> MSASFVPNGASLEDCHCNLFCLADLTGIKWKKYVWQGPTSAPILFPVTEEDPILSSFSRCLKADVLGVWRRDQRPGRRELWIFWWGEDPSFADLIHHDLSEEEDGVWENGLSYECRTLLFKAVHNLLERCLMNRNFVRIGKWFVKPYEKDEKPINKSEHLSCSFTFFLHGDSNVCTSVEINQHQPVYLLSEEHITLAQQSNSPFQVILCPFGLNGTLTGQAFKMSDSATKKLIGEWKQFYPISCCLKEMSEEKQEDMDWEDDSLAAVEVLVAGVRMIYPACFVLVPQSDIPTPSPVGSTHCSSSCLGVHQVPASTRDPAMSSVTLTPPTSPEEVQTVDPQSVQKWVKFSSVSDGFNSDSTSHHGGKIPRKLANHVVDRVWQECNMNRAQNKRKYSASSGGLCEEATAAKVASWDFVEATQRTNCSCLRHKNLKSRNAGQQGQAPSLGQQQQILPKHKTNEKQEKSEKPQKRPLTPFHHRVSVSDDVGMDADSASQRLVISAPDSQVRFSNIRTNDVAKTPQMHGTEMANSPQPPPLSPHPCDVVDEGVTKTPSTPQSQHFYQMPTPDPLVPSKPMEDRIDSLSQSFPPQYQEAVEPTVYVGTAVNLEEDEANIAWKYYKFPKKKDVEFLPPQLPSDKFKDDPVGPFGQESVTSVTELMVQCKKPLKVSDELVQQYQIKNQCLSAIASDAEQEPKIDPYAFVEGDEEFLFPDKKDRQNSEREAGKKHKVEDGTSSVTVLSHEEDAMSLFSPSIKQDAPRPTSHARPPSTSLIYDSDLAVSYTDLDNLFNSDEDELTPGSKKSANGSDDKASCKESKTGNLDPLSCISTADLHKMYPTPPSLEQHIMGFSPMNMNNKEYGSMDTTPGGTVLEGNSSSIGAQFKIEVDEGFCSPKPSEIKDFSYVYKPENCQILVGCSMFAPLKTLPSQYLPPIKLPEECIYRQSWTVGKLELLSSGPSMPFIKEGDGSNMDQEYGTAYTPQTHTSFGMPPSSAPPSNSGAGILPSPSTPRFPTPRTPRTPRTPRGAGGPASAQGSVKYENSDLYSPASTPSTCRPLNSVEPATVPSIPEAHSLYVNLILSESVMNLFKDCNFDSCCICVCNMNIKGADVGVYIPDPTQEAQYRCTCGFSAVMNRKFGNNSGLFLEDELDIIGRNTDCGKEAEKRFEALRATSAEHVNGGLKESEKLSDDLILLLQDQCTNLFSPFGAADQDPFPKSGVISNWVRVEERDCCNDCYLALEHGRQFMDNMSGGKVDEALVKSSCLHPWSKRNDVSMQCSQDILRMLLSLQPVLQDAIQKKRTVRPWGVQGPLTWQQFHKMAGRGSYGTDESPEPLPIPTFLLGYDYDYLVLSPFALPYWERLMLEPYGSQRDIAYVVLCPENEALLNGAKSFFRDLTAIYESCRLGQHRPVSRLLTDGIMRVGSTASKKLSEKLVAEWFSQAADGNNEAFSKLKLYAQVCRYDLGPYLASLPLDSSLLSQPNLVAPTSQSLITPPQMTNTGNANTPSATLASAASSTMTVTSGVAISTSVATANSTLTTASTSSSSSSNLNSGVSSNKLPSFPPFGSMNSNAAGSMSTQANTVQSGQLGGQQTSALQTAGISGESSSLPTQPHPDVSESTMDRDKVGIPTDGDSHAVTYPPAIVVYIIDPFTYENTDESTNSSSVWTLGLLRCFLEMVQTLPPHIKSTVSVQIIPCQYLLQPVKHEDREIYPQHLKSLAFSAFTQCRRPLPTSTNVKTLTGFGPGLAMETALRSPDRPECIRLYAPPFILAPVKDKQTELGETFGEAGQKYNVLFVGYCLSHDQRWILASCTDLYGELLETCIINIDVPNRARRKKSSARKFGLQKLWEWCLGLVQMSSLPWRVVIGRLGRIGHGELKDWSCLLSRRNLQSLSKRLKDMCRMCGISAADSPSILSACLVAMEPQGSFVIMPDSVSTGSVFGRSTTLNMQTSQLNTPQDTSCTHILVFPTSASVQVASATYTTENLDLAFNPNNDGADGMGIFDLLDTGDDLDPDIINILPASPTGSPVHSPGSHYPHGGDAGKGQSTDRLLSTEPHEEVPNILQQPLALGYFVSTAKAGPLPDWFWSACPQAQYQCPLFLKASLHLHVPSVQSDELLHSKHSHPLDSNQTSDVLRFVLEQYNALSWLTCDPATQDRRSCLPIHFVVLNQLYNFIMNML;> MKAQGETEESEKLSKMSSLLERLHAKFNQNRPWSETIKLVRQVMEKRVVMSSGGHQHLVSCLETLQKALKVTSLPAMTDRLESIARQNGLGSHLSASGTECYITSDMFYVEVQLDPAGQLCDVKVAHHGENPVSCPELVQQLREKNFDEFSKHLKGLVNLYNLPGDNKLKTKMYLALQSLEQDLSKMAIMYWKATNAGPLDKILHGSVGYLTPRSGGHLMNLKYYVSPSDLLDDKTASPIILHENNVSRSLGMNASVTIEGTSAVYKLPIAPLIMGSHPVDNKWTPSFSSITSANSVDLPACFFLKFPQPIPVSRAFVQKLQNCTGIPLFETQPTYAPLYELITQFELSKDPDPIPLNHNMRFYAALPGQQHCYFLNKDAPLPDGRSLQGTLVSKITFQHPGRVPLILNLIRHQVAYNTLIGSCVKRTILKEDSPGLLQFEVCPLSESRFSVSFQHPVNDSLVCVVMDVQDSTHVSCKLYKGLSDALICTDDFIAKVVQRCMSIPVTMRAIRRKAETIQADTPALSLIAETVEDMVKKNLPPASSPGYGMTTGNNPMSGTTTPTNTFPGGPITTLFNMSMSIKDRHESVGHGEDFSKVSQNPILTSLLQITGNGGSTIGSSPTPPHHTPPPVSSMAGNTKNHPMLMNLLKDNPAQDFSTLYGSSPLERQNSSSGSPRMEICSGSNKTKKKKSSRLPPEKPKHQTEDDFQRELFSMDVDSQNPIFDVNMTADTLDTPHITPAPSQCSTPPTTYPQPVPHPQPSIQRMVRLSSSDSIGPDVTDILSDIAEEASKLPSTSDDCPAIGTPLRDSSSSGHSQSTLFDSDVFQTNNNENPYTDPADLIADAAGSPSSDSPTNHFFHDGVDFNPDLLNSQSQSGFGEEYFDESSQSGDNDDFKGFASQALNTLGVPMLGGDNGETKFKGNNQADTVDFSIISVAGKALAPADLMEHHSGSQGPLLTTGDLGKEKTQKRVKEGNGTSNSTLSGPGLDSKPGKRSRTPSNDGKSKDKPPKRKKADTEGKSPSHSSSNRPFTPPTSTGGSKSPGSAGRSQTPPGVATPPIPKITIQIPKGTVMVGKPSSHSQYTSSGSVSSSGSKSHHSHSSSSSSSASTSGKMKSSKSEGSSSSKLSSSMYSSQGSSGSSQSKNSSQSGGKPGSSPITKHGLSSGSSSTKMKPQGKPSSLMNPSLSKPNISPSHSRPPGGSDKLASPMKPVPGTPPSSKAKSPISSGSGGSHMSGTSSSSGMKSSSGLGSSGSLSQKTPPSSNSCTASSSSFSSSGSSMSSSQNQHGSSKGKSPSRNKKPSLTAVIDKLKHGVVTSGPGGEDPLDGQMGVSTNSSSHPMSSKHNMSGGEFQGKREKSDKDKSKVSTSGSSVDSSKKTSESKNVGSTGVAKIIISKHDGGSPSIKAKVTLQKPGESSGEGLRPQMASSKNYGSPLISGSTPKHERGSPSHSKSPAYTPQNLDSESESGSSIAEKSYQNSPSSDDGIRPLPEYSTEKHKKHKKEKKKVKDKDRDRDRDKDRDKKKSHSIKPESWSKSPISSDQSLSMTSNTILSADRPSRLSPDFMIGEEDDDLMDVALIGN;> MAASSSGEKEKERLGGGLGVAGGNSTRERLLSALEDLEVLSRELIEMLAISRNQKLLQAGEENQVLELLIHRDGEFQELMKLALNQGKIHHEMQVLEKEVEKRDSDIQQLQKQLKEAEQILATAVYQAKEKLKSIEKARKGAISSEEIIKYAHRISASNAVCAPLTWVPGDPRRPYPTDLEMRSGLLGQMNNPSTNGVNGHLPGDALAAGRLPDVLAPQYPWQSNDMSMNMLPPNHSSDFLLEPPGHNKENEDDVEIMSTDSSSSSSESD;> MAAVDIRDNLLGISWVDSSWIPILNSGSVLDYFSERSNPFYDRTCNNEVVKMQRLTLEHLNQMVGIEYILLHAQEPILFIIRKQQRQSPAQVIPLADYYIIAGVIYQAPDLGSVINSRVLTAVHGIQSAFDEAMSYCRYHPSKGYWWHFKDHEEQDKVRPKAKRKEEPSSIFQRQRVDALLLDLRQKFPPKFVQLKPGEKPVPVDQTKKEAEPIPETVKPEEKETTKNVQQTVSAKGPPEKRMRLQ;> MGEPQQVSALPPPPMQYIKEYTDENIQEGLAPKPPPPIKDSYMMFGNQFQCDDLIIRPLESQGIERLHPMQFDHKKELRKLNMSILINFLDLLDILIRSPGSIKREEKLEDLKLLFVHVHHLINEYRPHQARETLRVMMEVQKRQRLETAERFQKHLERVIEMIQNCLASLPDDLPHSEAGMRVKTEPMDADDSNNCTGQNEHQRENSGHRRDQIIEKDAALCVLIDEMNERP;> MQREEKQLEASLDALLSQVADLKNSLGSFICKLENEYGRLTWPSVLDSFALLSGQLNTLNKVLKHEKTPLFRNQVIIPLVLSPDRDEDLMRQTEGRVPVFSHEVVPDHLRTKPDPEVEEQEKQLTTDAARIGADAAQKQIQSLNKMCSNLLEKISKEERESESGGLRPNKQTFNPTDTNALVAAVAFGKGLSNWRPSGSSGPGQAGQPGAGTILAGTSGLQQVQMAGAPSQQQPMLSGVQMAQAGQPGKMPSGIKTNIKSASMHPYQR;> MASAGVAAGRQAEDVLPPTSDQPLPDTKPLPPPQPPPVPAPQPQQSPAPRPQSPARAREEENYSFLPLVHNIIKCMDKDSPEVHQDLNALKSKFQEMRKLISTMPGIHLSPEQQQQQLQSLREQVRTKNELLQKYKSLCMFEIPKE;> MAEKFDHLEEHLEKFVENIRQLGIIVSDFQPSSQAGLNQKLNFIVTGLQDIDKCRQQLHDITVPLEVFEYIDQGRNPQLYTKECLERALAKNEQVKGKIDTMKKFKSLLIQELSKVFPEDMAKYRSIRGEDHPPS;> MATYSLANERLRALEDIEREIGAILQNAGTVILELSKEKTNERLLDRQAAAFTASVQHVEAELSAQIRYLTQVATGQPHEGSSYSSRKDCQMALKRVDYARLKLSDVARTCEQMLEN;> MAPVQLENHQLVPPGGGGGGSGGPPSAPAPPPPGAAVAAAAAAAASPGYRLSTLIEFLLHRAYSELMVLTDLLPRKSDVERKIEIVQFASRTRQLFVRLLALVKWANNAGKVEKCAMISSFLDQQAILFVDTADRLASLARDALVHARLPSFAIPYAIDVLTTGSYPRLPTCIRDKIIPPDPITKIEKQATLHQLNQILRHRLVTTDLPPQLANLTVANGRVKFRVEGEFEATLTVMGDDPDVPWRLLKLEILVEDKETGDGRALVHSMQISFIHQLVQSRLFADEKPLQDMYNCLHSFCLSLQLEVLHSQTLMLIRERWGDLVQVERYHAGKCLSLSVWNQQVLGRKTGTASVHKVTIKIDENDVSKPLQIFHDPPLPASDSKLVERAMKIDHLSIEKLLIDSVHARAHQKLQELKAILRGFNANENSSIETALPALVVPILEPCGNSECLHIFVDLHSGMFQLMLYGLDQATLDDMEKSVNDDMKRIIPWIQQLKFWLGQQRCKQSIKHLPTISSETLQLSNYSTHPIGNLSKNKLFIKLTRLPQYYIVVEMLEVPNKPTQLSYKYYFMSVNAADREDSPAMALLLQQFKENIQDLVFRTKTGKQTRTNAKRKLSDDPCPVESKKTKRAGEMCAFNKVLAHFVAMCDTNMPFVGLRLELSNLEIPHQGVQVEGDGFSHAIRLLKIPPCKGITEETQKALDRSLLDCTFRLQGRNNRTWVAELVFANCPLNGTSTREQGPSRHVYLTYENLLSEPVGGRKVVEMFLNDWNSIARLYECVLEFARSLPDIPAHLNIFSEVRVYNYRKLILCYGTTKGSSISIQWNSIHQKFHISLGTVGPNSGCSNCHNTILHQLQEMFNKTPNVVQLLQVLFDTQAPLNAINKLPTVPMLGLTQRTNTAYQCFSILPQSSTHIRLAFRNMYCIDIYCRSRGVVAIRDGAYSLFDNSKLVEGFYPAPGLKTFLNMFVDSNQDARRRSVNEDDNPPSPIGGDMMDSLISQLQPPPQQQPFPKQPGTSGAYPLTSPPTSYHSTVNQSPSMMHTQSPGNLHAASSPSGALRAPSPASFVPTPPPSSHGISIGPGASFASPHGTLDPSSPYTMVSPSGRAGNWPGSPQVSGPSPAARMPGMSPANPSLHSPVPDASHSPRAGTSSQTMPTNMPPPRKLPQRSWAASIPTILTHSALNILLLPSPTPGLVPGLAGSYLCSPLERFLGSVIMRRHLQRIIQQETLQLINSNEPGVIMFKTDALKCRVALSPKTNQTLQLKVTPENAGQWKPDELQVLEKFFETRVAGPPFKANTLIAFTKLLGAPTHILRDCVHIMKLELFPDQATQLKWNVQFCLTIPPSAPPIAPPGTPAVVLKSKMLFFLQLTQKTSVPPQEPVSIIVPIIYDMASGTTQQADIPRQQNSSVAAPMMVSNILKRFAEMNPPRQGECTIFAAVRDLMANLTLPPGGRP;> MDVSGQETDWRSTAFRQKLVSQIEDAMRKAGVAHSKSSKDMESHVFLKAKTRDEYLSLVARLIIHFRDIHNKKSQASVSDPMNALQSLTGGPAAGAAGIGMPPRGPGQSLGGMGSLGAMGQPMSLSGQPPPGTSGMAPHSMAVVSTATPQTQLQLQQVALQQQQQQQQFQQQQQAALQQQQQQQQQQQFQAQQSAMQQQFQAVVQQQQQLQQQQQQQQHLIKLHHQNQQQIQQQQQQLQRIAQLQLQQQQQQQQQQQQQQQQALQAQPPIQQPPMQQPQPPPSQALPQQLQQMHHTQHHQPPPQPQQPPVAQNQPSQLPPQSQTQPLVSQAQALPGQMLYTQPPLKFVRAPMVVQQPPVQPQVQQQQTAVQTAQAAQMVAPGVQMITEALAQGGMHIRARFPPTTAVSAIPSSSIPLGRQPMAQVSQSSLPMLSSPSPGQQVQTPQSMPPPPQPSPQPGQPSSQPNSNVSSGPAPSPSSFLPSPSPQPSQSPVTARTPQNFSVPSPGPLNTPVNPSSVMSPAGSSQAEEQQYLDKLKQLSKYIEPLRRMINKIDKNEDRKKDLSKMKSLLDILTDPSKRCPLKTLQKCEIALEKLKNDMAVPTPPPPPVPPTKQQYLCQPLLDAVLANIRSPVFNHSLYRTFVPAMTAIHGPPITAPVVCTRKRRLEDDERQSIPSVLQGEVARLDPKFLVNLDPSHCSNNGTVHLICKLDDKDLPSVPPLELSVPADYPAQSPLWIDRQWQYDANPFLQSVHRCMTSRLLQLPDKHSVTALLNTWAQSVHQACLSAA;> MCDLRRPAAGGMMDLAYVCEWEKWSKSTHCPSVPLACAWSCRNLIAFTMDLRSDDQDLTRMIHILDTEHPWDLHSIPSEHHEAITCLEWDQSGSRLLSADADGQIKCWSMADHLANSWESSVGSLVEGDPIVALSWLHNGVKLALHVEKSGASSFGEKFSRVKFSPSLTLFGGKPMEGWIAVTVSGLVTVSLLKPSGQVLTSTESLCRLRGRVALADIAFTGGGNIVVATADGSSASPVQFYKVCVSVVSEKCRIDTEILPSLFMRCTTDLNRKDKFPAITHLKFLARDMSEQVLLCASSQTSSIVECWSLRKEGLPVNNIFQQISPVVGDKQPTILKWRILSATNDLDRVSAVALPKLPISLTNTDLKVASDTQFYPGLGLALAFHDGSVHIVHRLSLQTMAVFYSSAAPRPVDEPAMKRPRTAGPAVHLKAMQLSWTSLALVGIDSHGKLSVLRLSPSMGHPLEVGLALRHLLFLLEYCMVTGYDWWDILLHVQPSMVQSLVEKLHEEYTRQTAALQQVLSTRILAMKASLCKLSPCTVTRVCDYHTKLFLIAISSTLKSLLRPHFLNTPDKSPGDRLTEICTKITDVDIDKVMINLKTEEFVLDMNTLQALQQLLQWVGDFVLYLLASLPNQGSLLRPGHSFLRDGTSLGMLRELMVVIRIWGLLKPSCLPVYTATSDTQDSMSLLFRLLTKLWICCRDEGPASEPDEALVDECCLLPSQLLIPSLDWLPASDGLVSRLQPKQPLRLQFGRAPTLPGSAATLQLDGLARAPGQPKIDHLRRLHLGACPTEECKACTRCGCVT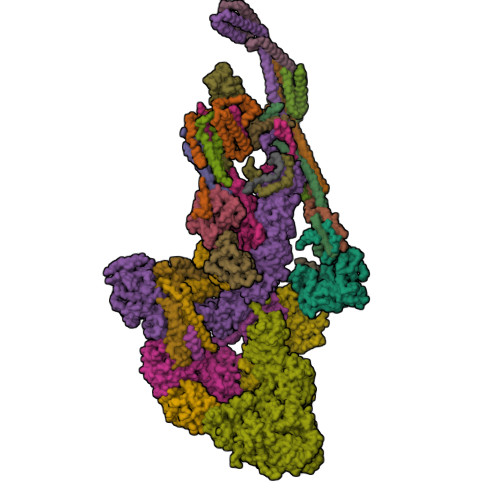MLKSPNRTTAVKQWEQRWIKNCLAVEGRGPDACVTSRASEEAPAFVQLGPQSTHHSPRTPRSLDHLHPEDRP;> MSGVRAVRISIESACEKQVHEVGLDGTETYLPPLSMSQNLARLAQRIDFSQGSGSEEEEAAGTEGDAQEWPGAGSSADQDDEEGVVKFQPSLWPWDSVRNNLRSALTEMCVLYDVLSIVRDKKFMTLDPVSQDALPPKQNPQTLQLISKKKSLAGAAQILLKGAERLTKSVTENQENKLQRDFNSELLRLRQHWKLRKVGDKILGDLSYRSAGSLFPHHGTFEVIKNTDLDLDKKIPEDYCPLDVQIPSDLEGSAYIKVSIQKQAPDIGDLGTVNLFKRPLPKSKPGSPHWQTKLEAAQNVLLCKEIFAQLSREAVQIKSQVPHIVVKNQIISQPFPSLQLSISLCHSSNDKKSQKFATEKQCPEDHLYVLEHNLHLLIREFHKQTLSSIMMPHPASAPFGHKRMRLSGPQAFDKNEINSLQSSEGLLEKIIKQAKHIFLRSRAAATIDSLASRIEDPQIQAHWSNINDVYESSVKVLITSQGYEQICKSIQLQLNIGVEQIRVVHRDGRVITLSYQEQELQDFLLSQMSQHQVHAVQQLAKVMGWQVLSFSNHVGLGPIESIGNASAITVASPSGDYAISVRNGPESGSKIMVQFPRNQCKDLPKSDVLQDNKWSHLRGPFKEVQWNKMEGRNFVYKMELLMSALSPCLL;> MEAPPVTMMPVTGGTINMMEYLLQGSVLDHSLESLIHRLRGLCDNMEPETFLDHEMVFLLKGQQASPFVLRARRSMDRAGAPWHLRYLGQPEMGDKNRHALVRNCVDIATSENLTDFLMEMGFRMDHEFVAKGHLFRKGIMKIMVYKIFRILVPGNTDSTEALSLSYLVELSVVAPAGQDMVSDDMKNFAEQLKPLVHLEKIDPKRLM;> MGVTCVSQMPVAEGKSVQQTVELLTRKLEMLGAEKQGTFCVDCETYHTAASTLGSQGQTGKLMYVMHNSEYPLSCFALFENGPCLIADTNFDVLMVKLKGFFQSAKASKIETRGTRYQYCDFLVKVGTVTMGPSARGISVEVEYGPCVVASDCWSLLLEFLQSFLGSHTPGAPAVFGNRHDAVYGPADTMVQYMELFNKIRKQQQVPVAGIR;> MADRLTQLQDAVNSLADQFCNAIGVLQQCGPPASFNNIQTAINKDQPANPTEEYAQLFAALIARTAKDIDVLIDSLPSEESTAALQAASLYKLEEENHEAATCLEDVVYRGDMLLEKIQSALADIAQSQLKTRSGTHSQSLPDS;> MAQQRALPQSKETLLQSYNKRLKDDIKSIMDNFTEIIKTAKIEDETQVSRATQGEQDNYEMHVRAANIVRAGESLMKLVSDLKQFLILNDFPSVNEAIDQRNQQLRTLQEECDRKLITLRDEISIDLYELEEEYYSSSSSLCEANDLPLCEAYGRLDLDTDSADGLSAPLLASPEPSAGPLQVAAPAHSHAGGPGPTEHA;> METQLQSIFEEVVKTEVIEEAFPGMFMDTPEDEKTKLISCLGAFRQFWGGLSQESHEQCIQWIVKFIHGQHSPKRISFLYDCLAMAVETGLLPPRLVCESLINSDTLEWERTQLWALTFKLVRKIIGGVDYKGVRDLLKVILEKILTIPNTVSSAVVQQLLAAREVIAYILERNACLLPAYFAVTEIRKLYPEGKLPHWLLGNLVSDFVDTFRPTARINSICGRCSLLPVVNNSGAICNSWKLDPATLRFPLKGLLPYDKDLFEPQTALLRYVLEQPYSRDMVCNMLGLNKQHKQRCPVLEDQLVDLVVYAMERSETEEKFDDGGTSQLLWQHLSSQLIFFVLFQFASFPHMVLSLHQKLAGRGLIKGRDHLMWVLLQFISGSIQKNALADFLPVMKLFDLLYPEKEYIPVPDINKPQSTHAFAMTCIWIHLNRKAQNDNSKLQIPIPHSLRLHHEFLQQSLRNKSLQMNDYKIALLCNAYSTNSECFTLPMGALVETIYGNGIMRIPLPGTNCMASGSITPLPMNLLDSLTVHAKMSLIHSIATRVIKLAHAKSSVALAPALVETYSRLLVYMEIESLGIKGFISQLLPTVFKSHAWGILHTLLEMFSYRMHHIQPHYRVQLLSHLHTLAAVAQTNQNQLHLCVESTALRLITALGSSEVQPQFTRFLSDPKTVLSAESEELNRALILTLARATHVTDFFTGSDSIQGTWCKDILQTIMSFTPHNWASHTLSCFPGPLQAFFKQNNVPQESRFNLKKNVEEEYRKWKSMSNENDIITHFSMQGSPPLFLCLLWKMLLETDHINQIGYRVLERIGARALVAHVRTFADFLVYEFSTSAGGQQLNKCIEILNDMVWKYNIVTLDRLILCLAMRSHEGNEAQVCYFIIQLLLLKPNDFRNRVSDFVKENSPEHWLQNDWHTKHMNYHKKYPEKLYFEGLAEQVDPPVQIQSPYLPIYFGNVCLRFLPVFDIVIHRFLELLPVSKSLETLLDHLGGLYKFHDRPVTYLYNTLHYYEMHLRDRAFLKRKLVHAIIGSLKDNRPQGWCLSDTYLKCAMNAREENPWVPDDTYYCRLIGRLVDTMAGKSPGPFPNCDWRFNEFPNPAAHALHVTCVELMALAVSGKEVGNALLNVVLKSQPLVPRENITAWMNAIGLIITALPEPYWIVLHDRIVSVISSPSLTSETEWVGYPFRLFDFTACHQSYSEMSCSYTLALAHAVWHHSSIGQLSLIPKFLTEVLLPIVKTEFQLLYVYHLVGPFLQRFQQERTRCMIEIGVAFYDMLLNVDQCSTHLNYMDPICDFLYHMKYMFTGDSVKEQVEKIICNLKPALKLRLRFITHISKMEPAAVPPQAMNSGSPAPQSNQVPVSLPVTQ;> MKVVNLKQAILQAWKERWSDYQWAINMKKFFPKGATWDILNLADALLEQAMIGPSPNPLILSYLKYAISSQMVSYSSVLTAISKFDDFSRDLCVQALLDIMDMFCDRLSCHGKAEECIGLCRALLSALHWLLRCTAASAERLREGLEAGTPAAGEKQLAMCLQRLEKTLSSTKNRALLHIAKLEEASSWTAIEHSLLKLGEILANLSNPQLRSQAEQCGTLIRSIPTMLSVHAEQMHKTGFPTVHAVILLEGTMNLTGETQSLVEQLTMVKRMQHIPTPLFVLEIWKACFVGLIESPEGTEELKWTAFTFLKIPQVLVKLKKYSHGDKDFTEDVNCAFEFLLKLTPLLDKADQRCNCDCTNFLLQECGKQGLLSEASVNNLMAKRKADREHAPQQKSGENANIQPNIQLILRAEPTVTNILKTMDADHSKSPEGLLGVLGHMLSGKSLDLLLAAAAATGKLKSFARKFINLNEFTTYGSEESTKPASVRALLFDISFLMLCHVAQTYGSEVILSESRTGAEVPFFETWMQTCMPEEGKILNPDHPCFRPDSTKVESLVALLNNSSEMKLVQMKWHEACLSISAAILEILNAWENGVLAFESIQKITDNIKGKVCSLAVCAVAWLVAHVRMLGLDEREKSLQMIRQLAGPLFSENTLQFYNERVVIMNSILERMCADVLQQTATQIKFPSTGVDTMPYWNLLPPKRPIKEVLTDIFAKVLEKGWVDSRSIHIFDTLLHMGGVYWFCNNLIKELLKETRKEHTLRAVELLYSIFCLDMQQVTLVLLGHILPGLLTDSSKWHSLMDPPGTALAKLAVWCALSSYSSHKGQASTRQKKRHREDIEDYISLFPLDDVQPSKLMRLLSSNEDDANILSSPTDRSMSSSLSASQLHTVNMRDPLNRVLANLFLLISSILGSRTAGPHTQFVQWFMEECVDCLEQGGRGSVLQFMPFTTVSELVKVSAMSSPKVVLAITDLSLPLGRQVAAKAIAAL;> MVPGSEGPARAGSVVADVVFVIEGTANLGPYFEGLRKHYLLPAIEYFNGGPPAETDFGGDYGGTQYSLVVFNTVDCAPESYVQCHAPTSSAYEFVTWLDGIKFMGGGGESCSLIAEGLSTALQLFDDFKKMREQIGQTHRVCLLICNSPPYLLPAVESTTYSGCTTENLVQQIGERGIHFSIVSPRKLPALRLLFEKAAPPALLEPLQPPTDVSQDPRHMVLVRGLVLPVGGGSAPGPLQSKQPVPLPPAAPSGATLSAAPQQPLPPVPPQYQVPGNLSAAQVAAQNAVEAAKNQKAGLGPRFSPITPLQQAAPGVGPPFSQAPAPQLPPGPPGAPKPPPASQPSLVSTVAPGSGLAPTAQPGAPSMAGTVAPGGVSGPSPAQLGAPALGGQQSVSNKLLAWSGVLEWQEKPKPASVDANTKLTRSLPCQVYVNHGENLKTEQWPQKLIMQLIPQQLLTTLGPLFRNSRMVQFHFTNKDLESLKGLYRIMGNGFAGCVHFPHTAPCEVRVLMLLYSSKKKIFMGLIPYDQSGFVNGIRQVITNHKQVQQQKLEQQQRGMGGQQAPPGLGPILEDQARPSQNLLQLRPPQPQPQGTVGASGATGQPQPQGTAQPPPGAPQGPPGAASGPPPPGPILRPQNPGANPQLRSLLLNPPPPQTGVPPPQASLHHLQPPGAPALLPPPHQGLGQPQLGPPLLHPPPAQSWPAQLPPRAPLPGQMLLSGGPRGPVPQPGLQPSVMEDDILMDLI;> MADVINVSVNLEAFSQAISAIQALRSSVSRVFDCLKDGMRNKETLEGREKAFIAHFQDNLHSVNRDLNELERLSNLVGKPSENHPLHNSGLLSLDPVQDKTPLYSQLLQAYKWSNKLQYHAGLASGLLNQQSLKRSANQMGVSAKRRPKAQPTTLVLPPQYVDDVISRIDRMFPEMSIHLSRPNGTSAMLLVTLGKVLKVIVVMRSLFIDRTIVKGYNENVYTEDGKLDIWSKSNYQVFQKVTDHATTALLHYQLPQMPDVVVRSFMTWLRSYIKLFQAPCQRCGKFLQDGLPPTWRDFRTLEAFHDTCRQ;> MAAPLGGMFSGQPPGPPQAPPGLPGQASLLQAAPGAPRPSSSTLVDELESSFEACFASLVSQDYVNGTDQEEIRTGVDQCIQKFLDIARQTECFFLQKRLQLSVQKPEQVIKEDVSELRNELQRKDALVQKHLTKLRHWQQVLEDINVQHKKPADIPQGSLAYLEQASANIPAPLKPT;> MAASQQQASAASSAAGVSGPSSAGGPGPQQQPQPPAQLVGPAQSGLLQQQQQDFDPVQRYKMLIPQLKESLQTLMKVAAQNLIQNTNIDNGQKSSDGPIQRFDKCLEEFYALCDQLELCLRLAHECLSQSCDSAKHSPTLVPTATKPDAVQPDSLPYPQYLAVIKAQISCAKDIHTALLDCANKVTGKTPAPPAGPGGTL;> MSTPPLAASGMAPGPFAGPQAQQAAREVNTASLCRIGQETVQDIVYRTMEIFQLLRNMQLPNGVTYHTGTYQDRLTKLQDNLRQLSVLFRKLRLVYDKCNENCGGMDPIPVEQLIPYVEEDGSKNDDRAGPPRFASEERREIAEVNKKLKQKNQQLKQIMDQLRNLIWDINAMLAMRN;> MAAAVAMETDDAGNRLRFQLELEFVQCLANPNYLNFLAQRGYFKDKAFVNYLKYLLYWKDPEYAKYLKYPQCLHMLELLQYEHFRKELVNAQCAKFIDEQQILHWQHYSRKRMRLQQALAEQQQQNNTSGK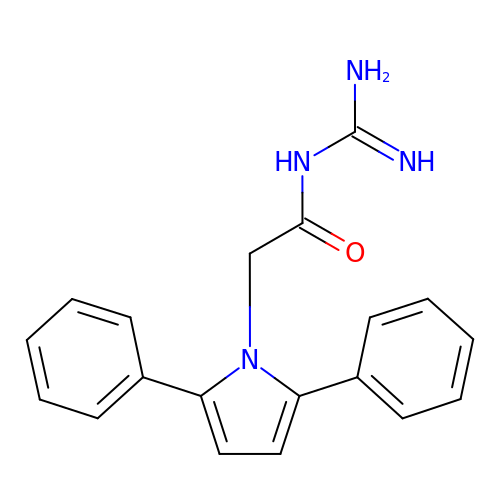N-[amino(imino)methyl]-2-(2,5-diphenyl-1H-pyrrol-1-yl)acetamide | C19 H18 N4 O | WVLDNAVUCUAGDP-UHFFFAOYSA-N> ARTKQTA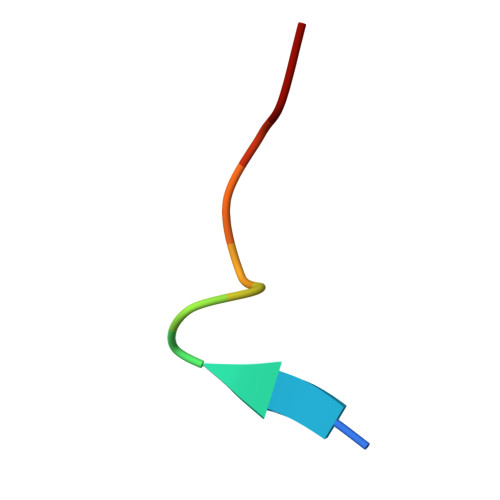RKSY structures of the Mep2 transceptors from S. cerevisiae and C. albicans. function as ammonium receptors/sensors in fungal development. a central channel for the transport of ammonium. non-phosphorylated, with channels that are closed on the cytoplasmic side.

structure using data to 3.4 Å resolution. region bridges the CTR and the main body of Mep2. Why then does this mutant appear to be constitutively active? to be disrupted by the incoming substrate to open the channel.

> MSGQFTGTGTGGDVFKVDLNEQFDRADMVWIGTASVLVWIMIPGVGLLYSGISRKKHALSLMWAALMAACVAAFQWFWWGYSLVFAHNGSVFLGTLQNFCLKDVLGAPSIVKTVPDILFCLYQGMFAAVTAILMAGAGCERARLGPMMVFLFIWLTVVYCPIAYWTWGGNGWLVSLGALDFAGGGPVHENSGFAALAYSLWLGKRHDPVAKGKVPKYKPHSVSSIVMGTIFLWFGWYGFNGGSTGNSSMRSWYACVNTNLAAATGGLTWMLVDWFRTGGKWSTVGLCMGAIAGLVGITPAAGYVPVYTSVIFGIVPAIICNFAVDLKDLLQIDDGMDVWALHGVGGFVGNFMTGLFAADYVAMIDGTEIDGGWMNHHWKQLGYQLAGSCAVAAWSFTVTSIILLAMDRIPFLRIRLHEDEEMLGTDLAQIGEYAYYADDDPEHHHHHH>[4x]EIPLKYGATNEGKRQDPAMQKFRDNRLGAFIHWGLYAIPGGEWNGKVYGGAAEWLKSWAKVPADEWLKLMDQWNPTKFDAKKWAKMAKEMGTKYVKITTKH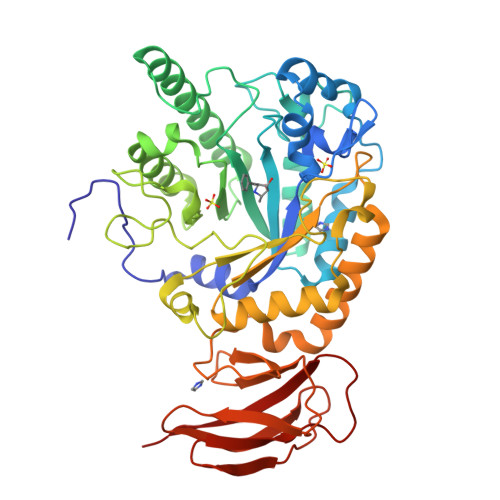HEGFCLWPSKYTKYTVANTPYKRDILGELVKAYNDEGIDVHFYFSVMDWSNPDYRYDIKSKEDSIAFSRFLEFTDNQLKELATRYPTVKDFWFDGTWDASVKKNGWWTAHAEQMLKELVPGVAINSRLRADDKGKRHFDSNGRLMGDYESGYERRLPDPVKDLKVTQWDWEACMTIPENQWGYHKDWSLSYVKTPIEVIDRIVHAVSMGGNMVVNFGPQADGDFRPEEKAMATAIGKWMNRYGKAVYACDYAGFEKQDWGYYTRGKNDEVYMVVFNQPYSERLIVKTPKGITVEKATLLTTGEDITVVETTRNEYNVSVPKKNPGEPYVIQLKVRAAK1[2-CHLORO-4-METHOXY-PHENYL-OXYMETHYL]-4-[2,6-DICHLORO-PHENYL-OXYMETHYL]-BENZENE 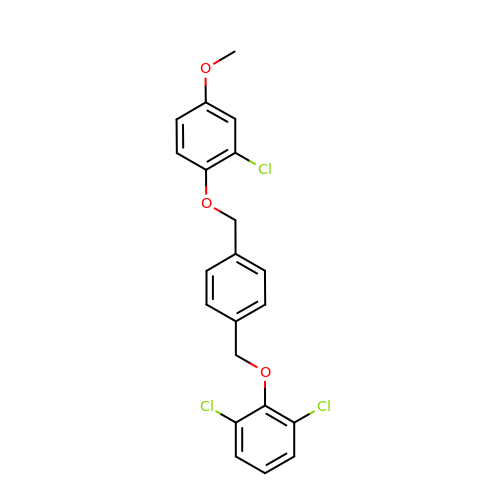| C21 H17 Cl3 O3 | XXMDDBVNWRWNCW-UHFFFAOYSA-N> AEIGGDHGYNATNIAAGQTSGAVTQIGPAVMGMVRRAIPNLIAFDICGVQPMNSPTGQVFALRAVYGKDPVAAGAKEAFHPMYGPDAMFSGQGAAKKFPALAASTQTTVGDIYTHFFQETGTVYLQASVQVTIDAGATDAAKLDAEIKKQMEAGALVEIAEGMATSIAELQEGFNGSTDNPWNEMGFRIDKQVIEAKSRQLKAAYSIELAQDLRAVHGMDADAELSGILATEIMLEINREVVDWINYSAQVGKSGMTLTPGSKAGVFDFQDPIDIRGARWAGESFKALLFQIDKEAVEIARQTGRGEGNFIIASRNVVNVLASVDTGISYAAQGLATG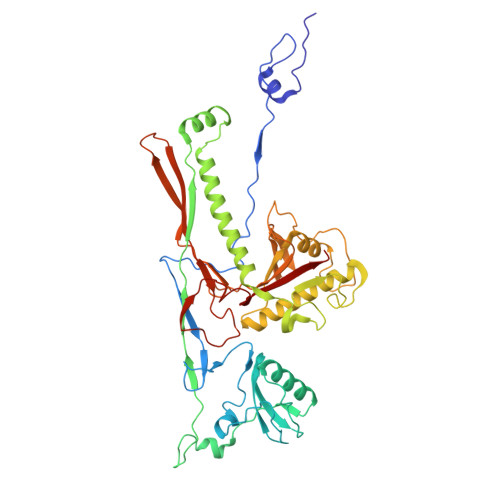FSTDTTKSVFAGVLGGKYRVYIDQYAKQDYFTVGYKGPNEMDAGIYYAPYVALTPLRGSDPKNFQPVMGFKTRYGIGINPFAESAAQAPASRIQSGMPSILNSLGKNAYFRRVYVKGI> MSTSASGPEHEFVSKFLTLATLTEPKLPKSYTKPLKDVTN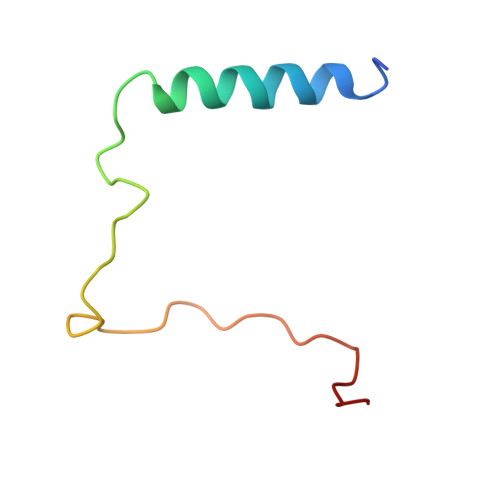LGVPLPTLKYKYKQNR>[2x]MHHHHHHHHHGGPISKILVANRSEIAIRVFRAANELGIKTVAIWAEEDKLALHRFKADESYQVGRGPHLARDLGPIESYLSIDEVIRVAKLSGADAIHPGYGLLSESPEFVDACNKAGIIFIGPKADTMRQLGNKVAARNLAISVGVPVVPATEPLPDDMAEVAKMAAAIGYPVMLKASWGGGGRGMRVIRSEADLAKEVTEAKREAMAAFGKDEVYLEKLVERARHVESQILGDTHGNVVHLFERDCSVQRRNQKVVERAPAPYLSEAQRQELAAYSLKIAGATNYIGAGTVEYLMDADTGKFYFIEVNPRIQVEHTVTEVVTGIDIVKAQIHILDGAAIGTPQSGVPNQEDIRLNGHALQCRVTTEDPEHNFIPDYGRITAYRSASGFGIRLDGGTSYSGAIITRYYDPLLVKVTAWAPNPLEAISRMDRALREFRIRGVATNLTFLEAIIGHPKFRDNSYTTRFIDTTPELFQQVKRQDRATKLLTYLADVTVNGHPEAKDRPKPLENAARPVVPYANGNGVKDGTKQLLDTLGPKKFGEWMRNEKRVLLTDTTMRDGHQSLLATRMRTYDIARIAGTYSHALPNLLSLECWGGATFDVSMRFLTEDPWERLALIREGAPNLLLQMLLRGANGVGYTNYPDNVVKYFVRQAAKGGIDLFRVFDCLNWVENMRVSMDAIAEENKLCEAAICYTGDILNSARPKYDLKYYTNLAVELEKAGAHIIAVKDMAGLLKPAAAKVLFKALREATGLPIHFHTHDTSGIAAATVLAAVEAGVDAVDAAMDALSGNTSQPCLGSIVEALSGSERDPGLDPAWIRRISFYWEAVRNQYAAFESDLKGPASEVYLHEMPGGQFTNLKEQARSLGLETRWHQVAQAYADANQMFGDIVKVAPSSKVVGDMALMMVSQDLTVADVVSP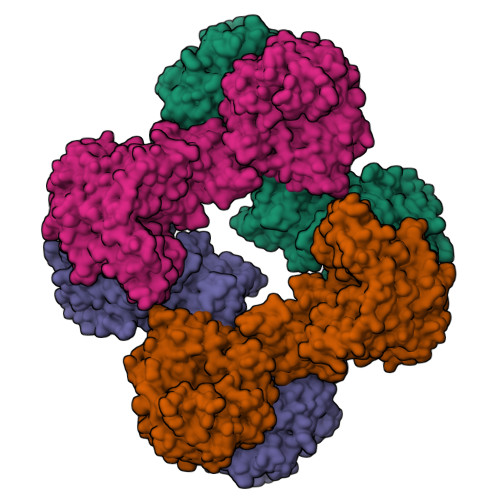DREVSFPESVVSMLKGDLGQPPSGWPEALQKKALKGEKPYTVRPGSLLKEADLDAERKVIEKKLEREVSDFEFASYLMYPKVFTDFALASDTYGPVSVLPTPAYFYGLADGEELFADIEKGKTLVIVNQAVSATDSQGMVTVFFELNGQPRRIKVPDRAHGATGAAVRRKAEPGNAAHVGAPMPGVISRVFVSSGQAVNAGDVLVSIEAMKMETAIHAEKDGTIAEVLVKAGDQIDAKDLLAVYGG> MSMAMSQSNRELVVDFLSYKLSQKGYSWSQFSDVEENRTEAPEGTESEAVKQALREAGDEFELRYRRAFSDLTSQLHITPGTAYQSFEQVVNELFRDGVNWGRIVAFFSFGGALCVESVD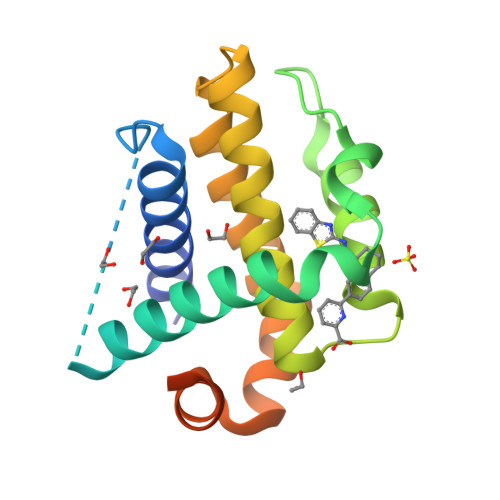KEMQVLVSRIAAWMATYLNDHLEPWIQENGGWDTFVELYGNNAAAESRKGQERLEHHHHHH> GSHMHAPYVEIIEQPKQRGMRFRYKCEGRSAGSIPGERSTDTTKTHPTIKINGYTGPGTVRISLVTKDPPHRPHPHELVGKDCRDGYYEADLCPDRSIHSFQNLGIQCVKKRDLEQAISQRIQTNNNPFHVPIEEQRGDYDLNAVRLCFQVTVRDPAGR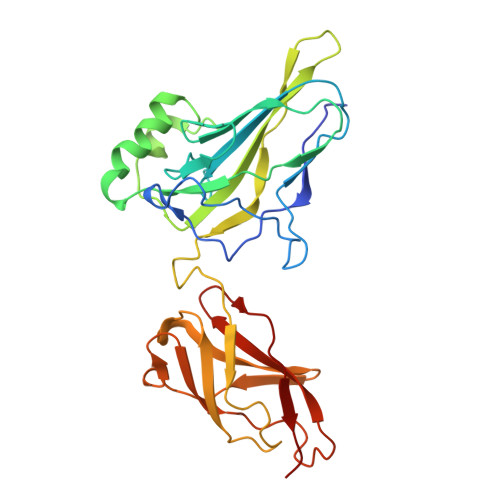PLLLTPVLSHPIFDNRAPNTAELKICRVNRNSGSCLGGDEIFLLCDKVQKEDIEVYFTGPGWEARGSFSQADVHRQVAIVFRTPPYADPSLQAPVRVSMQLRRPSDRELSEPMEFQYLPD> ASWSHPQFEKGASGAAESKPTPQSTFTGPIVVDPITRIEGHLRIMVEVENGKVKDAWSSSQLFRGLEIILKGRDPRDAQHFTQRACGVCTYVHALASSRCVDDAVKVSIPANARMMRNLVMASQYLHDHLVHFYHLHALDWVDVTAALKADPNKAAKLAASIAPARPGNSAKALKAVQDKLKAFVESGQLGIFTNAYFLGGHKAYYLPPEVDLIATAHYLEALHMQVKAASAMAILGGKNPHTQFTVVGGCSNYQGLTKNPLANYLALSKEVCQFVNECYIPDLLAVAGFYKDWGGIGGTSNYLAFGEFATDDSSPEKHLATSQFPSGVITGRDLGKVDNVDLGAIYEDVKYSWYAPGGDGKHPYDGVTDPKYTKLDDKDHYSWMKAPRYKGKAMEVGPLARTFIAYAKGQPDFKKVVDMVLGKLSV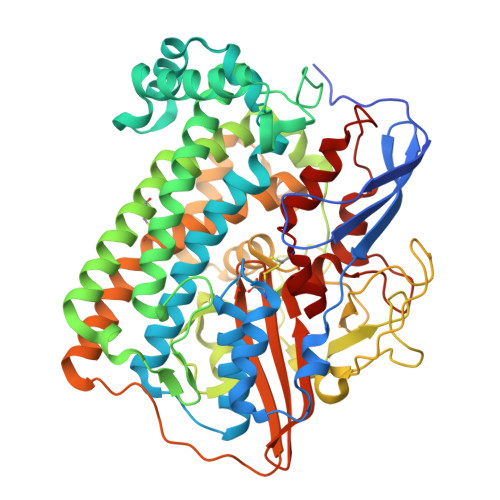PATALHSTLGRTAARGIETAIVCANMEKWIKEMADSGAKDNTLCAKWEMPEESKGVGLADAPRGALSHWIRIKGKKIDNFQLVVPSTWNLGPRGAQGDKSPVEEALIGTPIADPKRPVEILRTVHAFDPCIACGVH>[16x]MGFLTGKRALIVGVASKLSIASGIAAAMHREGAELAFTYQNDKLRGRVEEFASGWGSRPELCFPCDVADDSQIEAVFAALGKHWDGLDIIVHSVGFAPGDQLDGDFTAVTTREGFRIAHDISAYSFIALAKAGREMMKGRNGSLLTLSYLG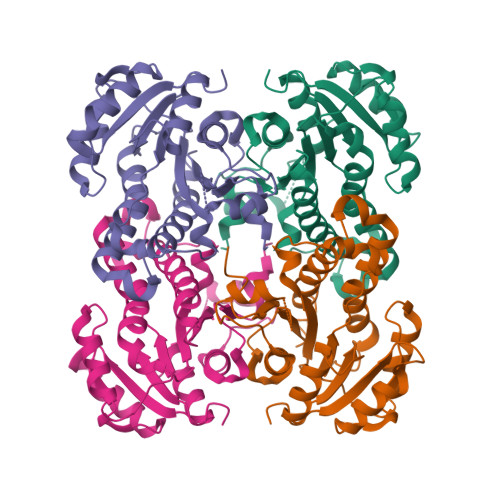AERTMPNYNVMGMAKASLEAGVRYLAGSLGAEGTRVNAVSAGPIRTLAASGIKSFRKMLAANERQTPLRRNVTIEEVGNAGAFLCSDLASGISGEILYVDGGFNTTAMGPLDDDLEHHHHHH> GIEETIDTVITNALQLSQPKPQKQPTAQSTPLTSGVNSQEVPALTAVETGASGQAVPSDVIETRHVVNYKTRSESTLESFFGRSACVTILEVENFNATTDADRKKQFTTWAITYTDTVQLRRKLEFFTYSRFDLEMTFVITERYYASNTGHARNQVYQLMYIPPGAPRPTAWDDYTWQSSSNPSVFYTYGSAPPRMSIPYVGIANAYSHFYDGFARVPLKDETVDSGDTYYGLVTINDFGTLAVRVVNEYNPARITSKIRVYMKPKHVRCWCPRPPRAVPYRGEGVDFKQDSITPLTAVENINTF;> SPNVEACGYSDRVRQITLGNSTITTQEAANAVVAYGEWPSYLDDKEANPIDAPTEPDVSSNRFYTLDSVQWKSTSRGWWWKLPDALKDMGMFGQNMYYHYLGRSGYTVHVQCNASKFHQGALGVFAIPEYVMACNTEAKTSYVSYVNANPGEKGGVFDNAYNPSAEASEGRKFAALDYLLGCGVLAGNAFVYPHQIINLRTNNSATLVLPYVNSLAIDCMAKHNNWGLVILPLCKLDYAPNSSTEIPITVTIAPMFTEFNGLRNITVPATQ;> GLP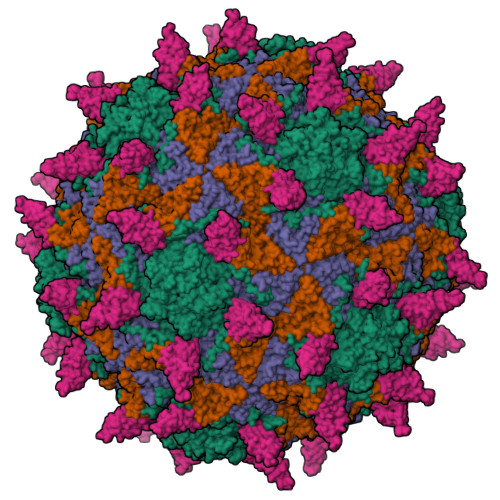TMLTPGSSQFLTSDDFQSPCALPNFDVTPPIHIPGEVFNMMELAEIDSMIPMNSVTGKANTMEMYPIPLDDKGSATPIFSISLSPASDKRLQYTMLGEILNYYTHWTGSLRFTFLFCGSMMATGKILLSYSPPGAKPPTTRKDAMLGTHIIWDLGLQSSCTMLAPWISNTVYRRCIKDDFTEGGYITCFYQTRIVVPSGTPTSMFMLAFVSACPDFSVRLLRDTNHISQRTLFARAQ;> QTSVSPSKVILPRGGSVLVTCSTSCDQPKLLGIETPLPKKELLLPGNNRKVYELSNVQEDSQPMCYSNCPDGQSTAKTFLTVYWT> DSEIDQLFRIFRALG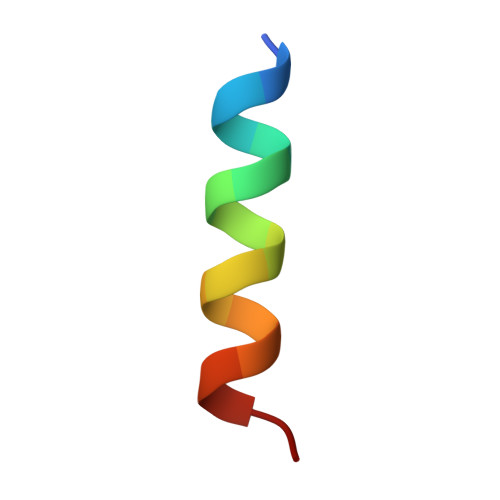TP2-(1-methyl-1H-1,2,3-triazol-5-yl)-5-((2-(pyridin-4-yl)pyrrolidin-1-yl)methyl)-1H-benzo[d]imidazole 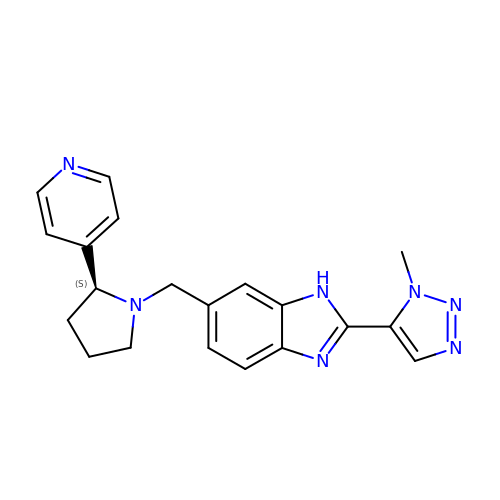| C20 H21 N7 | IEEIOQSIZMWGTQ-SFHVURJKSA-N>GAMAMSDLPIEFTELVDLMSLGISPQFLDFRSTTFESDHFVTVRETKDGTNSVAIVDLAKGNEVTRKNMGGDSAIMHPSQMVISVRANGTIVQIFNLETKSKLKSFTLDEPVIFWRWLSETTLGFVTARSILTSNVFDGNVNAKPQLLTLRHANLNNTQIINFVANKNLDWFAVVGILQENGRIAGRIQLFSKQRNISQAIDGHVAIFTNILLEGNGSTPVQVFVTGNRNATTGAGELRIIEIDHDASLPSQYQKETTDIFFPPDATNDFPIAVQVSEKYGIIYLLTKYGFIHLYELETGTNLFVNRITAESVFTAAPYN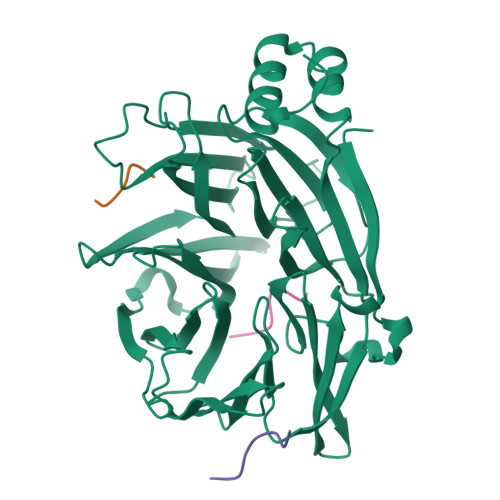HENGIACINKKGQVLAVEISTSQIVPYILNKLSNVALALIVATRGGLPGADDL[3x];>[9x]IPDLIDLDD> MGIMEAERKTTGWAARDPSGILSPYTYTLRETGPEDVNIRIICCGICHTDLHQTKNDLGMSNYP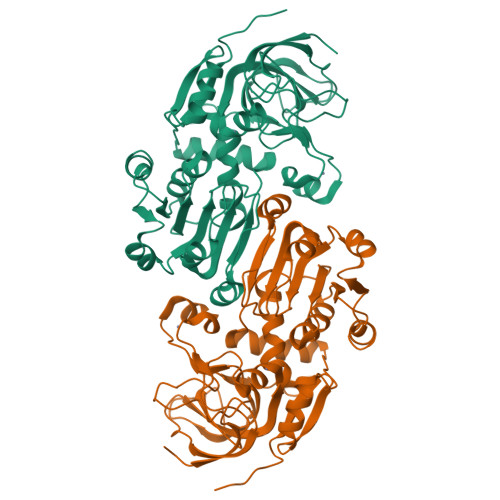MVPGHEVVGEVVEVGSDVSKFTVGDIVGVGCLVGCCGGCSPCERDLEQYCPKKIWSYNDVYINGQPTQGGFAKATVVHQKFVVKIPEGMAVEQAAPLLCAGVTVYSPLSHFGLKQPGLRGGILGLGGVGHMGVKIAKAMGHHVTVISSSNKKREEALQDLGADDYVIGSDQAKMSELADSLDYVIDTVPVHHALEPYLSLLKLDGKLILMGVINNPLQFLTPLLMLGRKVITGSFIGSMKETEEMLEFCKEKGLSSIIEVVKMDYVNTAFERLEKNDVRYRFVVDVEGSNLDA>AGDTKEQRILNHVLQHAEPGNAQSVLEAIDTYCEQKEWAMNVGDKKGKIVDAVIQEHQPSVLLELGAYCGYSAVRMARLLSPGARLITIEINPDCAAITQRMVDFAGVKDKVTLVVGASQDIIPQLKKKYDVDTLDMVFLDHWKDRYLPDTLLLEECGLL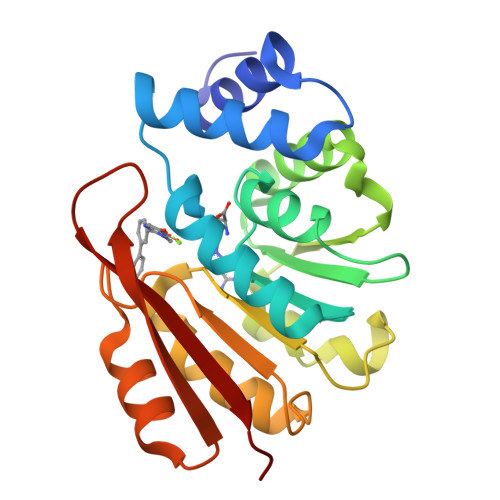RKGTVLLADNVICPGAPDFLAHVRGSSCFECTHYQSFLEYREVVDGLEKAIYKGP[2x]Hair cells have a characteristic morphology and harbor actin-filled stereocilia ‘staircases’ in which the stereocilia are coupled by protocadherin 15 (PCDH15) molecules from one stereocilium linked with cadherin 23 (CDH23) molecules from an adjacent stereocilium. Upon movement of the stereocilia induced by fluctuations of the surrounding fluid, the PCDH15-CDH23 ‘tip links’ trigger the opening of a mechano-electrical transduction (MET) ion channel at the stereocilia tips. PCDH15 belongs to the cadherin superfamily and consists of 11 extracellular cadherin (EC) domains, an extracellular linker (EL) domain, a single transmembrane (TM) helix and a cytoplasmic domain. Here we demonstrate that PCDH15 forms a robust complex with LHFPL5 and that the assembly is composed of 2 copies of each protein, thus providing concrete evidence that the composition of PCDH15 in the tip link is a dimer.

We discovered that a construct containing domains EC11 to CR, named PCDH151EC hereafter, when coexpressed with full length LHFPL5 yielded a well behaved complex. Two-dimensional (2D) classification of the resulting particles showed distinct secondary structure features of the EC11-EL and TM domains, indicating that this strategy was promising to result in a higher resolution reconstruction. A 3D reconstruction at ~4.5 Å resolution displayed three layers of density: a top layer formed by the EC11-EL domain, well fitted with the previously described crystal structure; a middle layer formed by the β-strand region of LHFPL5 and the extended C-terminal helix of the EL domain; and a bottom layer formed by the TM domains of PCDH15 and LHFPL5 (Figure 4—figure supplements 1 and 2c–e and Table 2). The resulting structure harbors an overall 2-fold symmetry, containing two copies of PCDH15 and LHFPL5. The density for the TM domain containing ten α-helices was well resolved, with some side chain features for bulky residues. Within the TM region there are extensive interactions between PCDH15 and LHFPL5. Each PCDH15 protomer makes more extensive interactions with one LHFPL5 protomer (1100 Å2 buried surface area, BSA) compared to the other (LHFPL5’, 270 Å2 BSA). We note that within the TM domains dimerization is primarily mediated by the interface of TM1 from LHFPL5 (487 Å2 BSA) together with the interaction of PCDH15 with TM1 of LHFPL5’. While there is a small interface of interactions between the 2-fold related PCDH15 TM helices (126 Å2 BSA), it likely is only a minor contributor to the stability of the complex. The extracellular domain of PCDH15 is situated ‘on top’ of the LHFPL5 β-sheet, but only minor direct interactions are apparent. While the crosslinking of the other residues is consistent with their close proximity in our model, the lack of a clearly defined periodicity indicates that the tip of the helices and the linker region are somewhat flexible.

>[2x]GQYDDHPPVFQKKFYIGGVSEDARMFASVLRVKATDRDTGNYSAMAYRLIIPPIKEGKEGFVVETYTGLIKTAMLFHNMRRSYFKFQVIATDDYGKGLSGKADVLVSVVNQLDMQVIVSNVPPTLVEKKIEDLTEILDRYVQEQIPGAKVVVESIGARRHGDAYSLEDYSKCDLTVYAIDPQTNRAIDRNELFKFLDGKLLDINKDFQPYYGEGGRILEIRTPEAVTSIKKRGESLGYTEGALLALAFIIILCCIPAILVVLVSYRQFKVRQAECTKTARIQSAMPAAKPAAPVPAAPAPPPPPPPPPPGAHLYEELGESAMHKYETALFESRLVPR;>GSGGRATMVKLLPAQEAAKIYHTNYVRNSRAVGVMWGTLTICFSVLVMALFIQPYWIGDSVSTPQAGYFGLFSYCVGNVLSSELICKGGPLDFSSIPSRAFKTAMFFVALAMFLIIGSIICFSLFFVCNTATVYKICAWMQLAAATGLMIGCLVYPDGWDSSEVRRMCGEQTGKYTLGHCTIRWAFMLAILSIGDALILSFLAFVLGYRQDKLLPDDYKADGNEEVFE[2x]>MSGSHHHHHHSGSMSERPSDLVVNRLVLFVVKGTATSTANTVKPLILLEELGVPHDIYVVEKVSAPWFSEINPHKMVPAI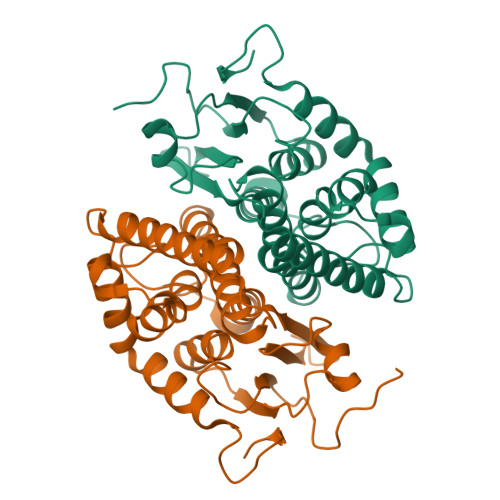LDRSPDGRDTLRAWESTSTLMYIADAYDKDGTFGGRNVQERSEINNWLTLHTAALGPTAKYWLYFYKLHPEKLPKTIEKLRSNITVQYDILERRLNEPGQQYLALKDRPTIADIATLPFAMKSTAELFGLEFEKWPKLQEWSVRMGEREAVKRAWQRVAGFGHGEKEYGMLEA[2x]>[2x]GIDPFTMTQTNRVIIFDTTLRDGEQSPGAAMTKEEKIRVARQLEKLGVDIIEAGFAAASPGDFEAVNAIAKTITKSTVCSLSRAIERDIRQAGEAVAPAPKKRIHTFIATSPIHMEYKLKMKPKQVIEAAVKAVKIAREYTDDVEFSCEDALRSEIDFLAEICGAVIEAGATT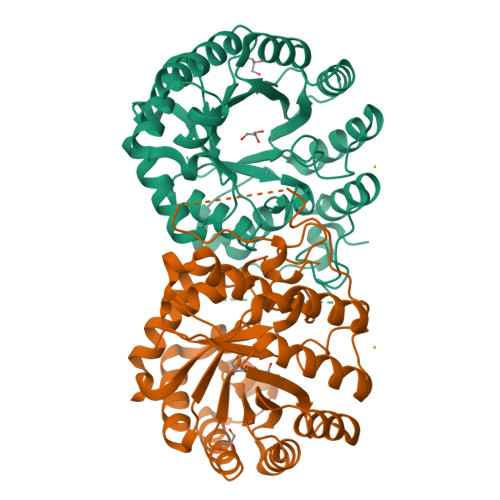INIPDTVGYSIPYKTEEFFRELIAKTPNGGKVVWSAHCHNDLGLAVANSLAALKGGARQVECTVNGLGERAGNASVEEIVMALKVRHDLFGLETGIDTTQIVPSSKLVSTITGYPVQPNKAIVGANAFSHESGIHQDGVLKHRETYEIMSAESVGWATNRLSLGKLSGRNAFKTKLADLGIELESEEALNAAFARFK>SMTATLRDAVAADLRSITEIYRESVLNGVATYEETPPSEAEMALRFSTITGNGYPYVVALDERGAVIGYAYASAFRNRTAYRFLVEDSIYLSPEARGKGIGKALLSELVGRCTALGFRQMIAVIGGAHPSSIAL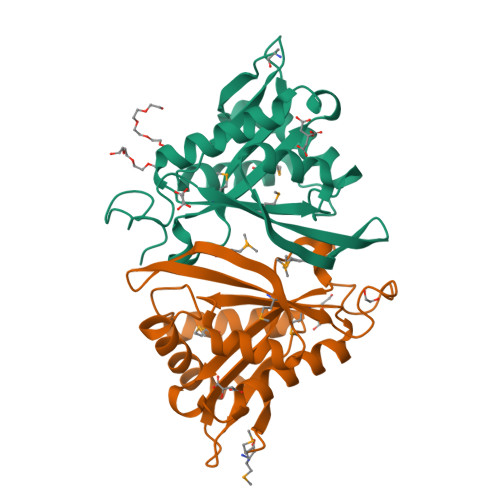HRALGFELQGLMKATGFKHGRWLDTAFMQRPLGEGTATKPTEGVYPDTLYRS[2x]>GSHMYLSKQLEFLFYVSSKEIIKKYTNYLKEYDLTYTGYIVLM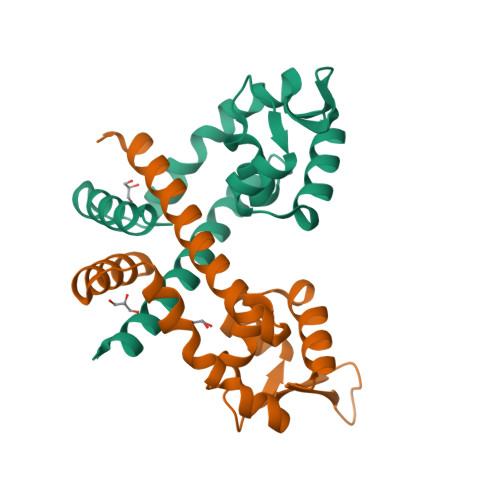AIENDEKLNIKKLGERVFLDSGTLTPLLKKLEKKDYVVRTREEKDERNLQISLTEQGKAIKSPLAEISVKVFNEFNISEREASDIINNLRNFVSKNF[2x]3'-DEOXY-3'-AMINOTHYMIDINE MONOPHOSPHATE | C10 H16 N3 O7 P | 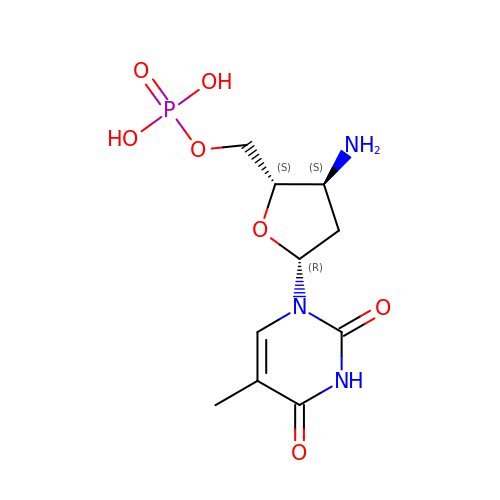BQZMHQZNZNBJNF-XLPZGREQSA-N>[2x]QDYNLVWQDEFDDGIGPDWVFETGMGYNGWGNNELQYYRRENAAVENGNLVITAK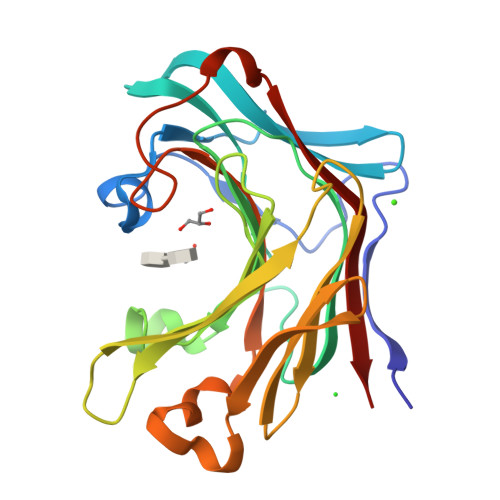HENFGGAQYTSARMKTQGRKSFKYGKIEARIALPSGQGLWPAFWMLGNNITSVSWPACGEIDIMSRINNALQTHGTIHWSDQNGDHASYGDDVGVSDPGQYHIYSVEWDANSIKWFVDGQQFNEVDISNGVNGTGEFQNEFFILLNMAVGGDWPGFDVDQSKLPAQMLVDYVRVYQKG>MEKNFVISDPRLPDNPIIFASDSFLELTEYSREEILGRNCRFLQGPETDQATVQKIRDAIRDQREITVQLINYTKSGKKFWNLFHLQPMRDQKGELQYFIGVQLDGEFIPNPLLGLDSTRTGHHHHHH[2x]

Phototropins are higher plant blue-light photoreceptors which regulate the response to excessive- or low-light levels, leading to, for instance, phototropism or chloro­plast movement, through two distinct light, oxygen or voltage-sensing (LOV) domains, LOV1 and LOV2. LOV domains, which belong to the larger Per–Arnt–Sim (PAS) family of small-molecule binding receptors, non-covalently bind the blue-light absorbing chromophore flavin mononucleotide (FMN). Under blue-light illumination, a covalent bond is formed between FMN and a nearby cysteine residue within microseconds, constituting a photoadduct. The formation of the photoadduct is associated with structural changes in the LOV1 and LOV2 domains, most notably the unfolding of the C-terminal helix of LOV2, Jα, which leads to the activation of a serine/threonine kinase domain.

Unexpectedly, we observed that, after a time corresponding to twice the relaxation time constant, the space group of the crystals changed from P43212 to P212121, suggesting that the in crystallo relaxation of the photoadduct population leads to a phase transition. In addition to this expected result, we observed an unanticipated phase transition, which occurs 70 to 80 s after the release of the PS equilibrium. This phase transition consists of the loss of a crystal symmetry element, which corresponds to the transition of the asymmetric unit from a monomer in the tetragonal space group P43212 to a dimer in the orthorhombic space group P212121. The non-crystallographic dimer is obtained from a crystallographic dimer whose molecules have slid apart. After the phase transition, the continuation of the ordering of the C-termini develops asymmetrically into distinct conformations and at different rates. While monomer A continues to fold in the α-helical conformation, which is completed within 130 s, monomer B refolds at a slower rate into a very different, hook-shaped conformation, which appears to be fully completed only after 1620 s. The difference in C-terminus conformation is coupled to the orientation of the side chain of a nearby bulky residue, W467, which rotates by ∼90° in order to accommodate the hook-shaped conformation of the C-terminus. Most importantly, we observe that residue W467, which belongs to a well conserved FWN sequence of residues found in LOV domains, acts as a gate discriminating between the two conformations of the C-terminus. The loss of this salt bridge may drive the sliding motion associated with the phase transition. In brief, we observed the appearance of a symmetry-breaking phenomenon during the in crystallo relaxation of the LOV2 photoadduct.> MDDLTIEILTDDADYDLQRFDCGEEALNLFLTTHLVRQHRNKILRAYILCRNTPERQVLGYYTLCGSCFERAALPSKSKQKKIPYKNIPSVTLGRLAIDRSLQGQGWGATLVAHAMNVVWSASLAVGIHGLFVEALNEKAHTFY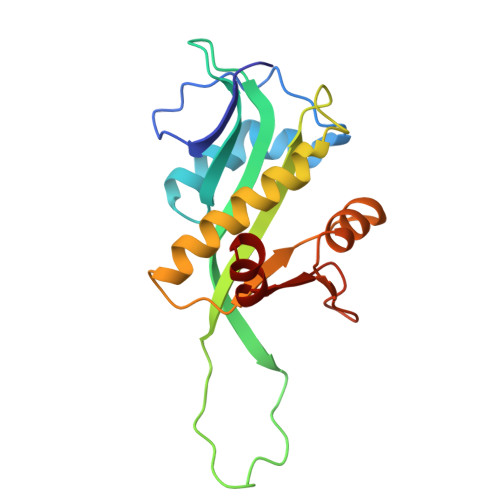KSLGFIPLVGENENALFFPTKSIELLFT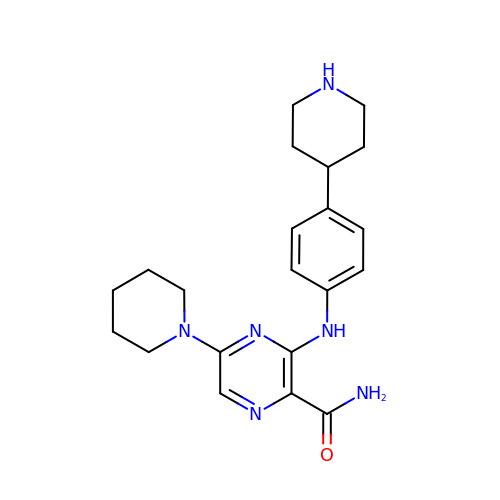5-(piperidin-1-yl)-3-[4-(piperidin-4-yl)anilino]pyrazine-2-carboxamide | C21 H28 N6 O | VGSQWWPMYSJONU-UHFFFAOYSA-N>[4x]GPAMCPTHADSLNNLANIKREQGNIEEAVRLYRKALEVFPEFAAAHSNLASVLQQQGKLQEALMHYKEAIRISPTFADAYSNMGNTLKEMQDVQGALQCYTRAIQINPAFADAHSNLASIHKDSGNIPEAIASYRTALKLKPDFPDAYCNLAHCLQIVCDWTDYDERMKKLVSIVADQLEKNRLPSVHPHHSMLYPLSHGFRKAIAERHGNLCLDKINVLHKPPYEHPKDLKLSDGRLRVGYVSSDFGNHPTSHLMQSIPGMHNPDKFEVFCYALSPDDGTNFRVKVMAEANHFIDLSQIPCNGKAADRIHQDGIHILVNM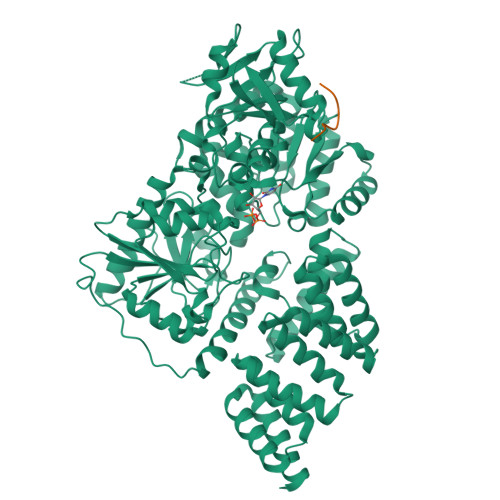NGYTKGARNELFALRPAPIQAMWLGYPGTSGALFMDYIITDQETSPAEVAEQYSEKLAYMPHTFFIGDHANMFPHLKKKAVIDFKSNGHIYDNRIVLNGIDLKAFLDSLPDVKIVKMKCPDGGDNADSSNTALNMPVIPMNTIAEAVIEMINRGQIQITINGFSISNGLATTQINNKAATGEEVPRTIIVTTRSQYGLPEDAIVYCNFNQLYKIDPSTLQMWANILKRVPNSVLWLLRFPAVGEPNIQQYAQNMGLPQNRIIFSPVAPKEEHVRRGQLADVCLDTPLCNGHTTGMDVLWAGTPMVTMPGETLASRVAASQLTCLGCLELIAKNRQEYEDIAVKLGTDLEYLKKVRGKVWKQRISSPLFNTKQYTMELERLYLQMWEHYAAGNKPDHMIKPVE;>[4x]FMPKYSI>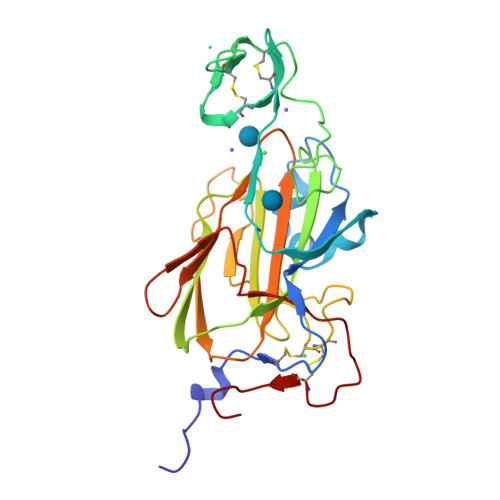 GLVPRGSHMSGATEACLPAGQRKSGMNINFYQYSLKDSSTYSNAAYMAYGYASKTKLGSVGGQTDISIDYNIPCVSSSGTFPCPQEDSYGNWGCKGMGACSNSQGIAYWSTDLFGFYTTPTNVTLEMTGYFLPPQTGSYTFSFATVDDSAILSVGGSIAFECCAQEQPPITSTNFTINGIKPWDGSLPTNITGTVYMYAGYYYPLKVVYSNAVSWGTLPISVELPDGTTVSDNFEGYVYSFDDDLSQSNCTIPDPSIH> GANAMAMASLINLTPHDVTVFDGDTPIASWPASGTFARIMEDVAAPAPMDTDQG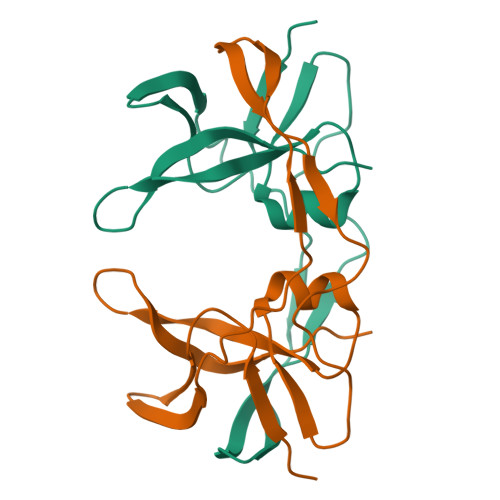FVPVSQVRYADTVDGLPGKVSGTAYLVSRVLAAAVPRDDLYFPLDEVRDATGRIIGCRALGQFDHSHTEERGDA> SEVGKSFKDRKMIEKMQEENRKDREKAAAKFREYFPNFVGEPKSKDILKLRLYEMQHGKCLYSGK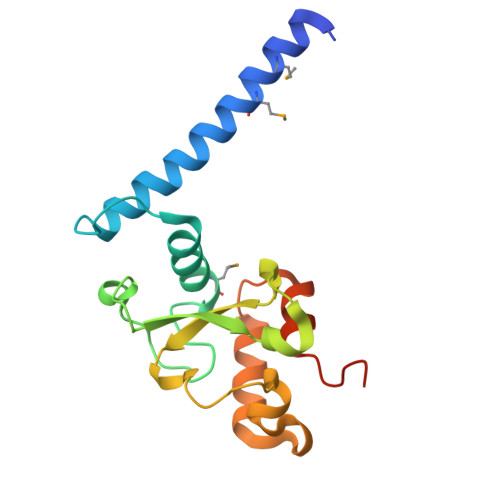EINLGRLNEKGYVEIDHALPFSRTWDDSFNNKVLVLGSENQNKGNQTPYEYFNGKDNSREWQEFKARVETSRFPRSKKQRILLQKFDEDGFKERNL3-Aminopropyl 2-deoxy-2-(4-phenyl-1,2,3-triazol-1-yl)-alpha-D-mannopyranoside 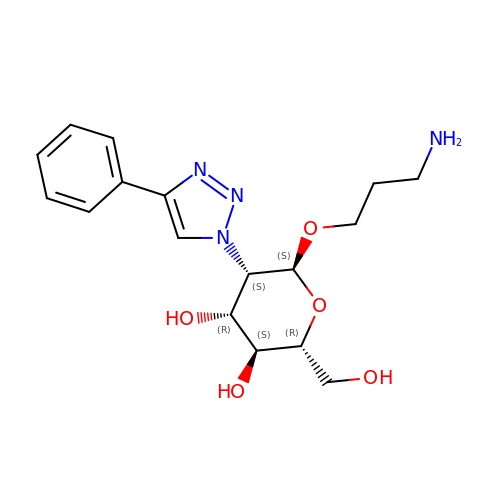| C17 H24 N4 O5 | XCUIOLRELJNONY-JJTUDDRGSA-N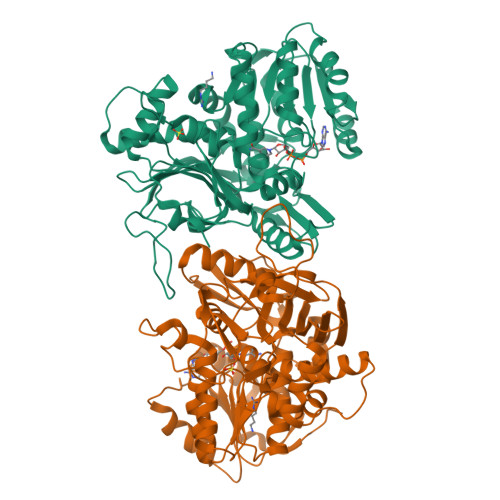>[2x]GPMGTDWPVYHRIDGPIVMIGFGSIGRGTLPLIERHFAFDRSKLVVIDPSDEARKLAEARGVRFIQQAVTRDNYRELLVPLLTAGPGQGFCVNLSVDTSSLDIMELARENGALYIDTVVEPWLGFYFDPDLKPEARSNYALRETVLAARRNKPGGTTAVSCCGANPGMVSWFVKQALVNLAADLGVTGEEPTTREEWARLAMDLGVKGIHIAARDTQRASFPKPFDVFVNTWSVEGFVSEGLQPAELGWGTFERWMPDNARGHDSGCGAGIYLLQPGANTRVRSWTPTAMAQYGFLVTHNESISIADFLTVRDAAGQAVYRPTCHYAYHPCNDAVLSLHEMFGSGKRQSDWRILDETEIVDGIDELGVLLYGHGKNAYWYGSQLSIEETRRIAPDQNATGLQVSSAVLAGMVWALENPNAGIVEADDLDFRRCLEVQTPYLGPVVGVYTDWTPLAGRPGLFPEDIDTSDPWQFRNVLVRD>GQVPEGYPANYAKAPRFKALIYYTQHAEEAHVQFAEQATTFFKKLNYGDGFVLDITTDFSKYPYEKLKEYNVIIMLNTSPNTKAERDAFEQYMENGGGWVGFHAAAYNDKNTHWPWFVKFLGGGVFYCNNWPPQPVLVEVDNEEHPVTKNLPASFVAPASEWYQWTPSPRQNKDVEVLLSLSPKNYPLGIKDVVNFGDFPIVWSNK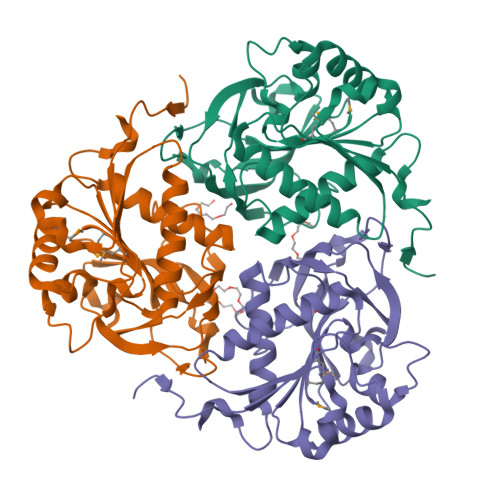NYRMIYLNMGHGDEEFIDGTQNLLLVNAFRWVVSKDKSGNPFLK[3x]> CGACG;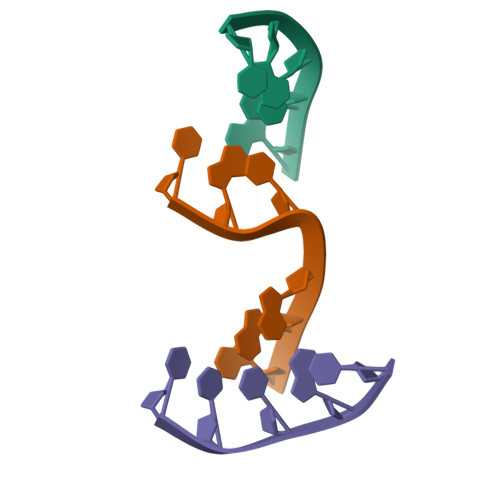> TCCGC;> CGTGGA> MVINQTFLQNNVMDKCNDKRKRGERDWDCPAEKDICISDRRYQLCMKELTNLVNNTRTHSHNDITFLKLNLKRKLMYDAAVEGDLLLKKNNYQYNKEFCKDIRWGLGDFGDIIMGTNMEGIGYSQVVENNLRSIFGTDEKAKQDRKQWWNESKEHIWRAMMFSLRSRLKEKFVWICKKDVTLKVEPQIYRWIREWGRDYMSELPKEQGKLNEKCASKLYYNNMAICMLPLCHDACKSYDQWITRKKKQWDVLSTKFSSVKKTQKIGTENIATAYDILKQELNGFKEATFENEINKRDNLYNHLCPCVVEEARKNTQENVKNVGSG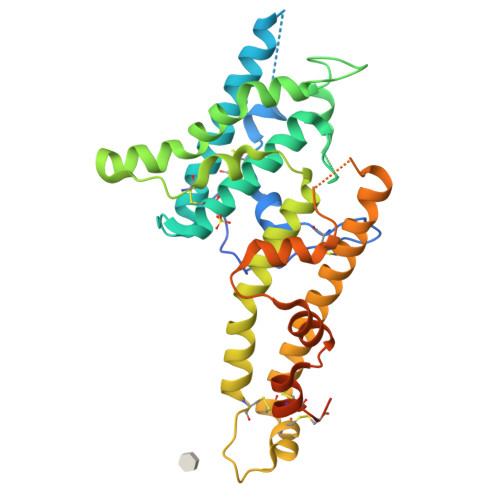VESKAASSNPITE> QQAGTNTAENHPQLQSQQCTTSGGCKPLSTKVVLDSNWRWVHSTSGYTNCYTGNEWDTSLCPDGKTCAANCALDGADYSGTYGITSTGTALTLKFVTGSNVGSRVYLMADDTHYQLLKLLNQEFTFDVDMSNLPCGLNGALYLSAMDADGGMSKYPGNKAGAKYGTGYCDSQCPKDIKFINGEANVGNWTETGSNTGTGSYGTCCSEMDIWEANNDAAAFTPHPCTTTGQTRC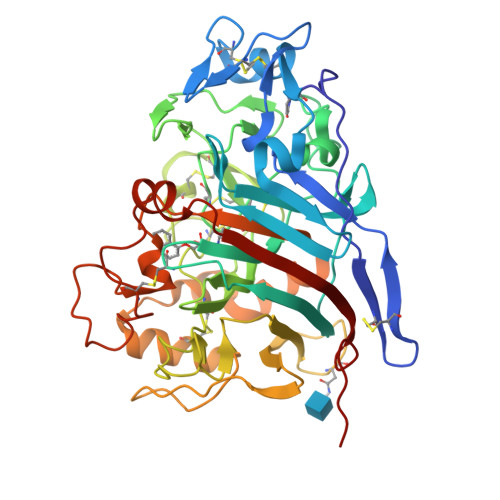SGDDCARNTGLCDGDGCDFNSFRMGDKTFLGKGMTVDTSKPFTVVTQFLTNDNTSTGTLSEIRRIYIQNGKVIQNSVANIPGVDPVNSITDNFCAQQKTAFGDTNWFAQKGGLKQMGEALGNGMVLALSIWDDHAANMLWLDSDYPTDKDPSAPGVARGTCATTSGVPSDVESQVPNSQVVFSNIKFGDIGSTFSGTS>[2x]AMAEAYQIQSNGDPQSKPLLELYVKASGIDARRIGADLFCQEFWMELYALYEIGVARVEVKTVNVNSEAFKKNFLGAQPPIMIEEEKELTYTDNREIEGRIFHLAKEFNVPLFEKDPSAEKRIENLYRNFKLFLRAKVEFDKGKKEPSRVE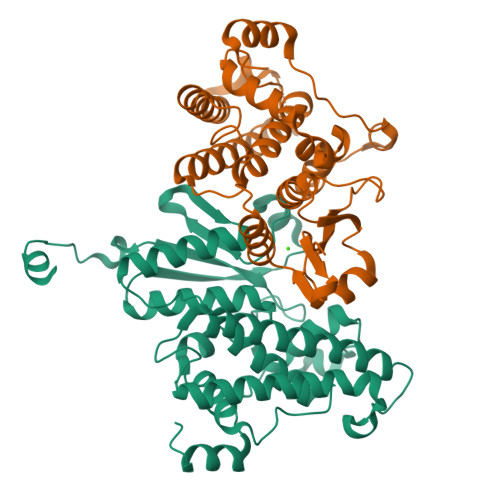DLPAQIKVHYNRVCEQLSNIDQLLSERKSRYLLGNSMTEYDCELMPRLHHIRIIGLSLLGFDIPHNFTHLWAYILTAYRTAAFIESCPADQDIIHHYKEQMNLFTNQRETLQSPTKTHTIPEKVLSDIRVKGLAPDVNVH> MIVSDIEANALLESVTKFHCGVIYDYSTAEYVSYRPSDFGAYLDALEAEVARGGLIVFHNGHKYDVPALTKLAKLQLNREFHLPRENCIDTLVLSRLIHSNLKDTDMGLLRSGKLPGALEAWGYRLGEMKGEYKDDFKRMLEEQGEEYVDGMEWWNFNEEMMDYNVQDVVVTKALLEKLLSDKHYFPPEIDFTDVGYTTFWSESLEAVDIEHRAAWLLAKQERNGFPFDTKAIEELYVELAARRSELLRKLTETFGSWYQPKGGTEMFCHPRTGKPLPKYPRIKTPKVGGIFKKPKNKAQREGREPCELDTREYVAGAPYTPVEHVVFNPSSRDHIQKKLQEAGWVPTKYTDK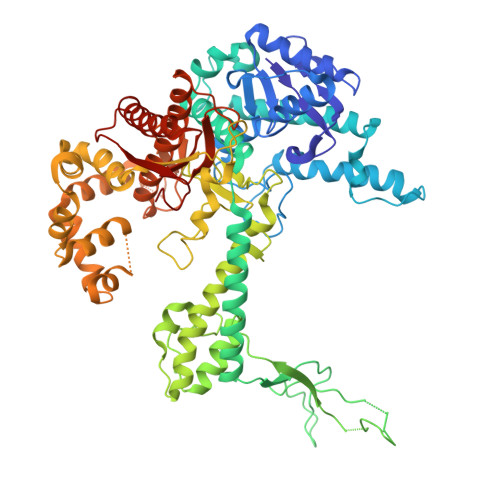GAPVVDDEVLEGVRVDDPEKQAAIDLIKEYLMIQKRIGQSAEGDKAWLRYVAEDGKIHGSVNPNGAVTGRATHAFPNLAQIPGVRSPYGEQCRAAFGAEHHLDGITGKPWVQAGIDASGLELRCLAHFMARFDNGEYAHEILNGDIHTKNQIAAELPTRDNAKTFIYGFLYGAGDEKIGQIVGAGKERGKELKKKFLENTPAIAALRESIQQTLVESSQWVAGEQQVKWKRRWIKGLDGRKVHVRSPHAALNTLLQSAGALICKLWIIKTEEMLVEKGLKHGWDGDFAYMAWVHDEIQVGCRTEEIAQVVIETAQEAMRWVGDHWNFRCLLDTEGKMGPNWAICH> AVPTVVGIPDGTAVVGRSFRVSIPTDLIASSGEIIKVSAAGKEALPSWLHWDPHSHILEGLPLDTDKGVHYISVSAARLGANGSHVPQTSSVFSIEVYPEDHNEPQSVRAASSDPGEVV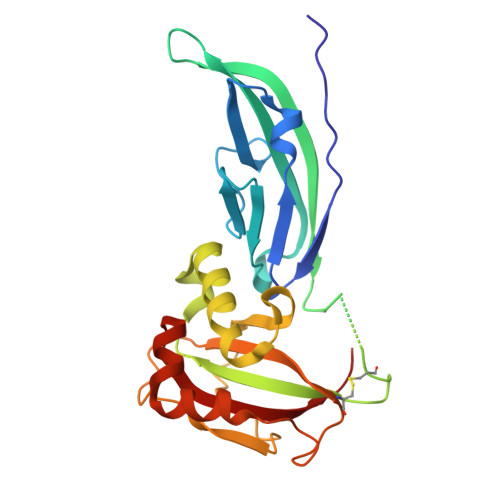PSACAADEPVTVLTVILDADLTKMTPKQRIDLLNRMQSFSEVELHNMKLVPVVNNRLFDMSAFMAGPGNAKKVVENGALLSWKLGCSLNQNSVPDIRGVETPAREGAMSAQLGYPVVGWHIANKKPT> ACPEDWGASSRTSLCFKLYAKGKHEKKTWFESRDFC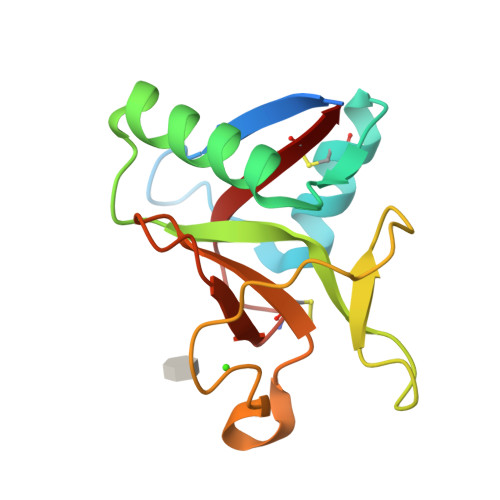RALGGDLASINNKEEQQTIWRLITASGSYHKLFWLGLTYGSPSEGFTWSDGSPVSYENWAYGEPNNYQNVEYCGELKGDPTMSWNDINCEHLNNWICQI> GPHMLEMPKEKYEPPDPRRMYTIMSSEEAANGKKSHWAELEISGKVRSLSASLWSLTHLTALHLSDNSLSRIPSDIAKLHNLVYLDLSSNKIRSLPAELGNMVSLRELHLNNNLLRVLPFELGKLFQLQTLGLKGNPLTQDILNLYQEPDGTRRLLNYLLDNLSGTAKRITTEQPPPRSWIMLQEPDRTRPTALFSVMCYNVLCDKYATRQLYGYCPSWALNWDYRKKAIIQEILSCNADIVSLQEVETEQYYSFFLVELKERGYNGFFSPKSRARTMSEQERKHVDGCAIFFKTEKFTLVQKHTVEFNQLAMANSEGSEAMLNRVMTKDNIGVAVLLELRKESIEMPSGKPHLGTEKQLILVANAHMHWDPEYSDVKLVQTMMFLSEVKNIIDKASRNLKSSVLGEFGTIPLVLCADLNSLPDSGVVEYLSTGGVETNHKDFKELRYNESLTNFSCHGKNGTTNGRITHGFKLQSAYESGLMPYTNYTFDFKGIIDYIFYSKPQLNTLGILGPLDHHWLVENNISGCPHPLIPSDHFSLFAQLELLLPFLPQVNGIHLPGRR;> GPHMLEPAATVDHSQRICEVWACNLDEEMKKIRQVIRKYNYVAMDTEFPGVVARPIGEFRSNADYQYQLLRCNVDLLKIIQLGLTFMNEQGEYPPGTSTWQFNFKFNLTEDMYAQDSIELLTTSGIQFKKHEEEGIETQYFAELLMTSGVVLCEGVKWLSFHSGYDFGYLIKILTNSNLPEEELDFFEILRLFFPVIYDVKYLMKSCKNLKGGLQEVAEQLELERIGPQHQAGSDSLLTGMAFFKMREMFFEDHIDDAKYCGHLYGLGSGSSYVQNGTGNAYEEEANKQS

The CCR4 and CAF1 deadenylases physically interact to form the CCR4-CAF1 complex and function as the catalytic core of the larger CCR4-NOT complex. Together, they are responsible for the eventual removal of the 3′-poly(A) tail from essentially all cellular mRNAs and consequently play a central role in the posttranscriptional regulation of gene expression. CCR4 belongs to the heterogeneous EEP (exonuclease-endonuclease-phosphatase) family of phosphoesterases, whereas CAF1 belongs to the DEDDh family of nucleases, which also comprises PARN and PAN2 (34,35). Consequently, CAF1 serves as a bridge between the NOT proteins and CCR4.

To characterize the catalytic core of the human CCR4-NOT complex, we coexpressed human CCR4a and CAF1a in E. coli, purified the complex (in the following named CCR4-CAF1) and determined a crystal structure at 3.3 Å resolution. All of the three protein domains, the CCR4 LRR domain (S29–S158), the CCR4 nuclease domain (I164–L545), and the CAF1 nuclease (Q10–L262), were clearly defined in the electron density, with the exception of some loops and disordered regions, which are not included in the model. Human CCR4 only contains a short N-terminal extension (M1–K28), which is followed by four and a half LRR repeats (LRR1 to LRR5) and two C-terminal α-helices that shield the hydrophobic residues of the last, incomplete repeat unit (LRR5). This N-terminal LRR domain of CCR4 binds the CAF1 nuclease in an oriented manner, whereas the C-terminal nuclease domain of CCR4 is connected to the LRR domain by a short linker (G159–R163) and fixed by crystal packing forces, apparently without specific contacts to the remainder of the complex. The linker is traceable in the electron density and assures that the CCR4 nuclease domain remains closely tethered, but nevertheless adaptable with respect to the CCR4 LRR domain and the CAF1 nuclease. The two active sites remain almost 50 Å apart and in an orientation that precludes them to work simultaneously on the same RNA 3′-end. In the interface, the hydrophobic surface of the first LRR repeat gets covered by hydrophobic residues from CAF1 α-helix α2 (C67 and L71) and by M107, as observed for the corresponding residues A215, F219 and I256 in S. cerevisiae. Importantly, the loop L(β2–α2) rearranges upon complex formation with the CCR4 LRR domain and folds into an additional turn of α-helix α2 and into the two β-strands βL1 and βL2, which pair with distinct β-strands from the CCR4 LRR domain. Difference electron density was observed in the active sites of both CCR4 and CAF1 and was interpreted by placing Mg2+ ions. However, due to the limited resolution of our crystal structure, we roughly positioned only a single Mg2+ ion to interpret the elongated difference electron density in CAF1.> MSSLKKILGLKGKGKKSKKLGIAPPPYEEDTSMEYAPSAPIDKSYFGVDEMDTYDPNQLRYEKFFFTVKMTVRSNRPFRTYSDVAAAVSHWDHMYIGMAGKRPFYKILAFL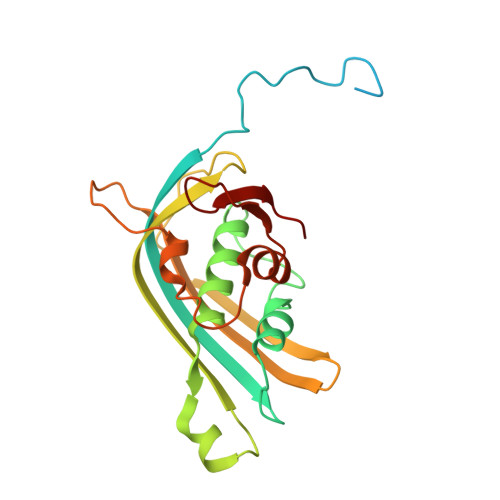GSSNLKATPAVLADQGQPEYHAHCEGRAYLPHRMGKTPPMLNVPEHFRRPFNIGLYKGTIELTMTIYDDESLEAAPMIWDHFNSSKFSDFREKALMFGLIVEKKASGAWVLDSISHFK[2-amino-1-(piperidin-4-ylmethyl)-1H-benzimidazol-6-yl](phenyl)methanone | C20 H22 N4 O | 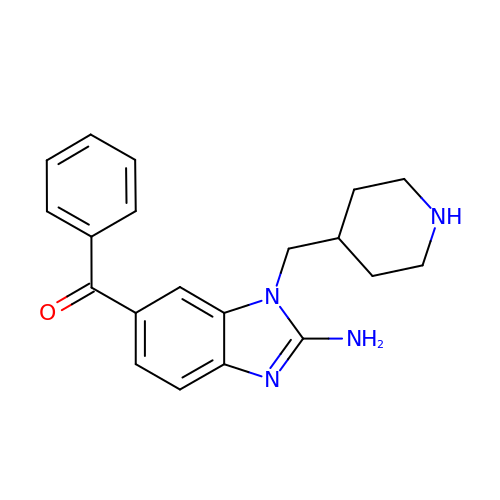CMCWMODUNMLBRJ-UHFFFAOYSA-N>[8x]AIVPTRELENVF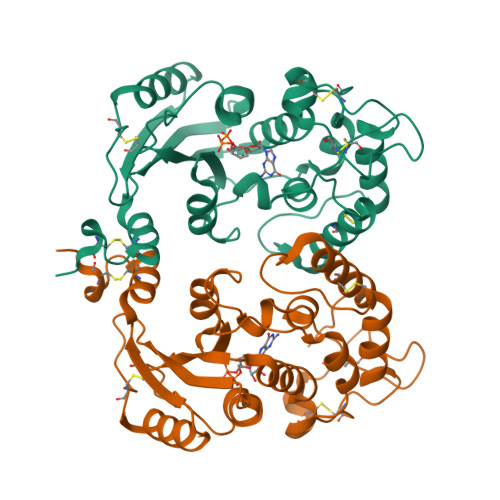LGRCKDYEITRYLDILPRVRSDCSALWKDFFKAFSFKNPCDLDLGSYKDFFTSAQQQLPKNKVMFWSGVYDEAHDYANTGRKYITLEDTLPGYMLNSLVWCGQRANPGFNEKVCPDFKTCPVQARESFWGMASSSYAHSAEGEVTYMVDGSNPKVPAYRPDSFFGKYELPNLTNKVTRVKVIVLHRLGEKIIEKCGAGSLLDLEKLVKAKHFAFDCVENPRAVLFLLCSDNPNARECRLAKRFYRIA>[3x]AMKPAQKGKTFSNVEIFDPPTNYRDPQVLYARPLELSDGTLLGTWENYSPEPPNVWFPIVKSKDGGKTWKEISKVKDTQNNWGLRYQPQLYELPRAFGKYPKGTVLCSGSSIPSDLSETLIEVYASRDKGYTWEFVSHVALGGEALPNPGLTPVWEPFLMTYKEKLILYYSDQRDNATHSQK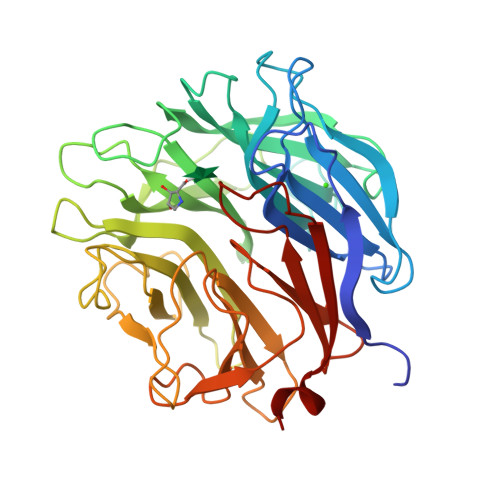LVHQTTTDLKKWSKVVDDTKYANYYARPGMPTVAKLPNNEYIYVYAYGGGPNPPAGSDYWFPVYYRLSKDPQKFLNKAHHQIVSNDGTTPAGSPYVVWTPYGGKNGTIVVSCGTRSEIFTNQALGDASAWKKWDVPQPTAYTRSLLTFQKDPDLLMIMGAGILPPAGGKNTVSASVVRLSEVMKS>SGQFELEILSMQNVNGELQNGNCCGGARNPGDRKCTRDECDTYFKVCLKEYQSRVTAGGPCSFGSGSTPVIGGNTFNLKASRGNDRNRIVLPFSFAWPRSYTLLVEAWDSSNDTVQPDSIIEKASHSGMINPSRQWQTLKQNTGVAHFEYQIRVTCDDYYYGFGCNKFCRPRDDFFGHYACDQNGNKTCMEGWMGPECNRAICRQGCSPKHGSCKLPGDCRCQYGWQGLYCDKCIPHPGCVHGICNEPWQCLCETNWGGQLCDKDLNYCGTHQPCLNGGTCSNTGPDKYQCSCPEGYSGPNCEIVDHHHHHH[2x]

Signals are initiated by extracellular interactions of the Notch receptor with Delta/Serrate/Lag-2 (DSL) ligands, whose structure is highly conserved throughout evolution. Here, we demonstrate that the N terminus of human Jagged-1 is a C2 phospholipid recognition domain that binds phospholipid bilayers in a calcium-dependent fashion. We expressed and solved the structure of a Notch ligand fragment consisting of the full N-terminal extension, the Notch-binding DSL domain, and the three adjacent EGF domains from human Jagged-1 (J-1N-EGF3). Our structure demonstrates that the N-terminal portion of Jagged-1 folds as a C2-phospholipid-recognition domain with strong structural, but not sequence, homology to the Munc13 C2B domain (root-mean-square deviation [rmsd] 2.7 Å versus Protein Data Bank 3KWT, 10% sequence identity; Figure 1B; Cho and Stahelin, 2006; Shin et al., 2010).

The C2 domain packs closely on top of the Notch-binding DSL domain without altering the structure of the DSL-EGF1-3 portion of the construct in comparison with our earlier structure for this region in isolation, and therefore extends the near-linear domain organization (Cordle et al., 2008a). Many missense mutations that affect this domain of J-1 cause Alagille syndrome, a developmental disorder that is usually associated with J-1 haploinsufficiency, and mapping these mutations onto our structure suggests that they destabilize the hydrophobic core and prevent correct folding of the C2 domain (Penton et al., 2012). Sequence alignments with other Notch ligands suggest that the C2 domain is present in all mammalian Notch ligands, with conserved residues mapping to those that play key structural roles, and residues exposed on the surface of the domain being more variable. Since the strongest structural homology of the J-1 C2 domain is to calcium-dependent phospholipid-binding domains (e.g., the Munc13-1 C2b domain; Shin et al., 2010), we investigated whether J-1N-EGF3 binds Ca2+. We first used a limited proteolysis assay, which showed that Ca2+ (but not Mg2+ or EDTA) protects the J-1N-EGF3 fragment (but not a J-1 fragment lacking the C2 domain) from tryptic digestion. This suggests the presence of previously unrecognized Ca2+-binding sites, occupancy of which increases the degree of structure in the C2 domain.> GPGSMIDDIYNKRILEFAGNMERIGQLAEPDAVATVHSKLCGSTVTVYLKMRDGVVTDFAHEVKACALGQASSSVMARNVIGATADELRAARDAMYRMLKENGPAPEGRFADMK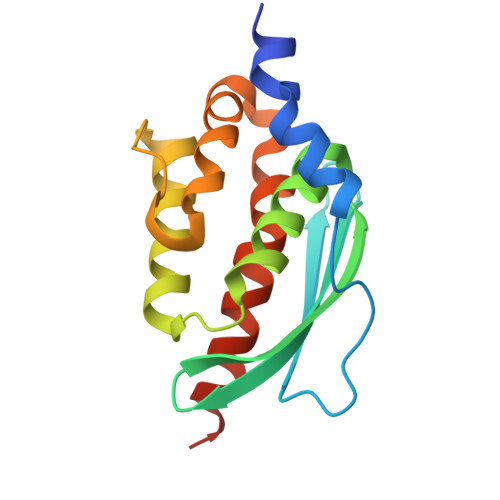YFEPVRDYKARHASTLLTFDAVADCIRQIEEKAKAA> MDEALIKDYHSIREQIDQYTKDMVLVMQHPTNCVKYINPGRLMHVVTSDGTDFGWGVIINFYERRPERNNPNPGWSPQESYVVEVLLRLSSDSGSVDSKLKDNQCIPAGIAPVTQKNDPGRWEVVPCLLSCMHGLSQIKL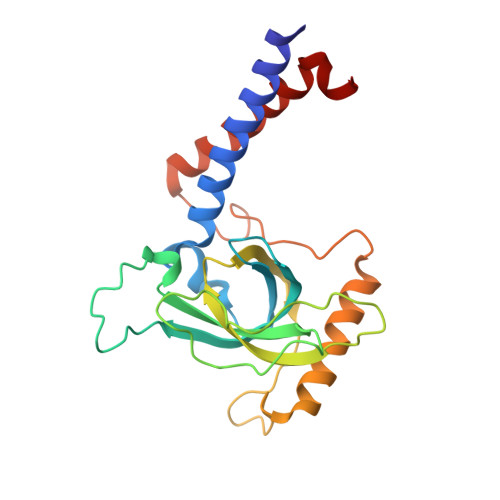HVPDKKSGGSMDDPETRRRVGKSLLEVQRRFEDGIPHMDPIENMHIRDVEFKKLLRKIEVLESRLVANPLHNS>[4x]MRIVPFGAAREVTGSAHLLLAGGRRVLLDCGMFQGKEEARNHAPFGFDPKEVDAVLLTHAHLDHVGRLPKLFREGYRGPVYAT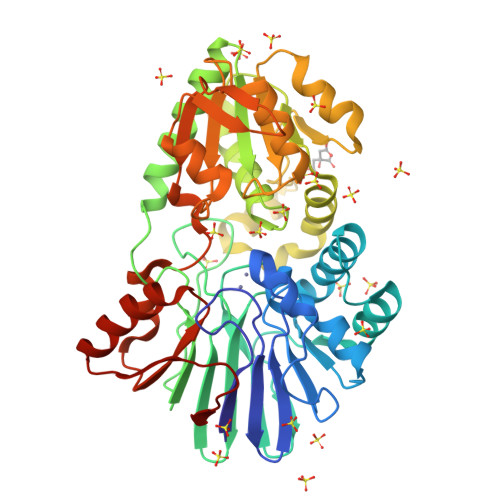RATVLLMEIVLEDALKVMDEPFFGPEDVEEALGHLRPLEYGEWLRLGALSLAFGQAGHLPGSAFVVAQGEGRTLVYSGDLGNREKDVLPDPSLPPLADLVLAEGTYGDRPHRPYRETVREFLEILEKTLSQGGKVLIPTFAVERAQEILYVLYTHGHRLPRAPIYLDSPMAGRVLSLYPRLVRYFSEEVQAHFLQGKNPFRPAGLEVVEHTEASKALNRAPGPMVVLAGSGMLAGGRILHHLKHGLSDPRNALVFVGYQPQGGLGAEIIARPPAVRILGEEVPLRASVHTLGGFQGHAGQDELLDWLQGEPRVVLVHGEEEKLLALGKLLALRGQEVSLARFGEGVPV>MVSTTETAEAEPVKKLEKVSKKQEEGLVTNKYKPKEPYVGRCLLNTRITGDQAPGETWHMVFSTEGEVPYREGQSIGVIADGEDKNGKPHKLRLYSIASSALGDFGDSKTVSLCVKRLVYTNDQGEVVKGVCSNFLCDLKPGAEVKITGP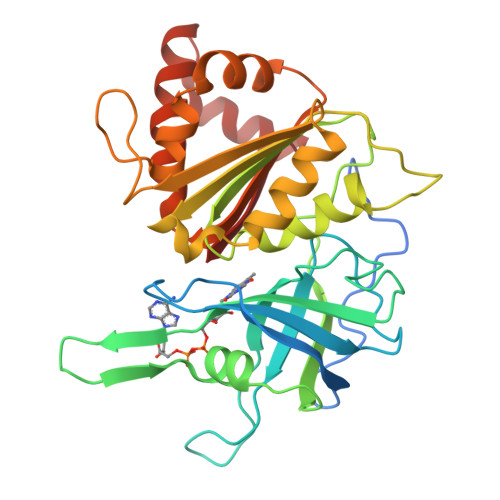VGKEMLMPKDPNATIIMLATGTGIAPFRSFLWKMFFEEHEDYKYTGLAWLFLGVPTSDTLLYKEELEKMKEMAPDNFRLDFAVSREQTNAAGEKMYIQTRMAEYKEELWELLKKDNTYVYMCGLKGMEKGIDDIMLDLAAKDGINWLDYKKQLKKSEQWNVEVY[2x]> XADVAGTSNRDFRGREQRLFNSEQ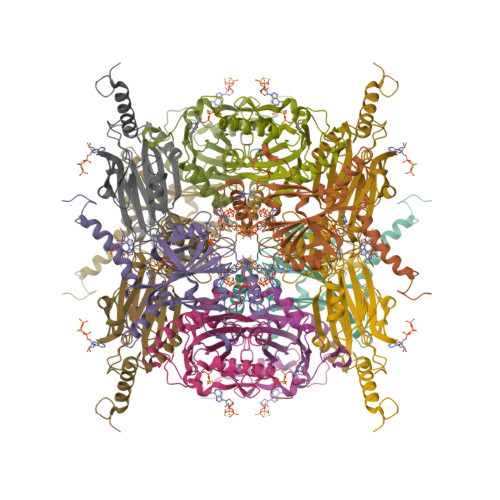YNYNNSLNGEVSVWVYAYYSDGSVLVINKNSQYKVGISETFKALKEYREGQHNDSYDEYEVNQSIYYPNGGDARKFHSNAKPRAIQIIFSPSVNVRTIKMAKGNAVSVPDEYLQRSHPWEATGIKYRKIKRDGEIVGYSHYFELPHEYNSISLAVSGVHKNPSSYNVGSAHNVMDVFQSCDLALRFCNRYWAELELVNHYISPNAYPYLDINNHSYGVALSNRQ> EDISEPPLHDFYCSRLLDLVFLLDGSSRLSEAEFEVLKAFVVDMMERLRISQKWVRVAVVEYHDGSHAYIGLKDRKRPSELRRIASQVKYAGSQ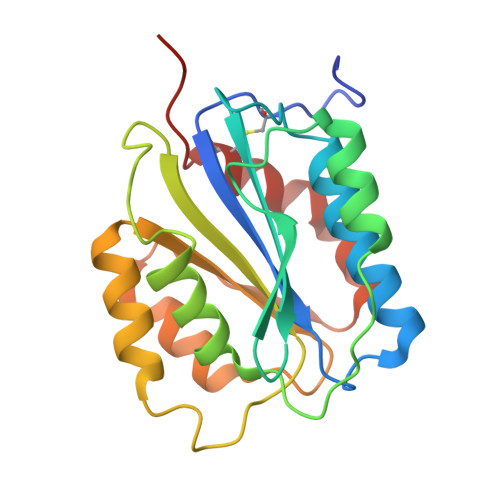VASTSEVLKYTLFQIFSKIDRPEASRIALLLMASQEPQRMSRNFVRYVQGLKKKKVIVIPVGIGPHANLKQIRLIEKQAPENKAFVLSSVDELEQQRDEIVSYLCDLAPEAPPPT> MHHHHHHAVRASEISRVYEAYPEKKATLYFLVLGFLALIVGSLFGPFQALNYGNVDAYPLLKRLLPFVQSYYQGLTLHGVLNAIVFTQLFAQAIMVYLPARELNMRPNMGLMWLSWWMAFIGLVVAALPLLANEATVLYTFYPPLKGHWAFYLGASVFVLSTWVSIYIVLDLWRRWKAANPGKVTPLVTYMAVVFWLMWFLASLGLVLEFVLFLLPWSFGLVEGVDPLVARTLFWWTGHPIVYFWLLPAYAIIYTILPKQAGGKLVSDPMARLAFLLFLLLSTPVGFHHQFADPGIDPTWKMIHSVLTLFVAVPSLMTAFTVAASLEFAGRLRGGRGLFGWIRALPWDNPAFVAPVLGLLGFIPGGAGGIVNASFTLDYVVHNTAWVPGHFHLQVASLVTLTAMGSLYWLLPNLTGKPISDAQRRLGLAVVWLWFLGMMIMAVGLHWAGLLNVPRRAYIAQVPDAYPHAAVPMVFNVLAGIVLLVALLLFIYGLFSVLLSRERKPELAEAPLPFAEVISGPEDRRLVLAMDRIGFWFAVAAILVVLAYGPTLVQLFGHLNPVPGWRLW;> MVDEHKAHKAILAYEKGWLAFSLAMLFVFIALIAYTLATHTAGVIPAGKLERVDPTTVRQEGPWADPAQAVVQTGPNQYTVYVLAFAFGYQPNPIEVPQGAEIVFKITSPDVIHGFHVEGTNINVEVLPGEVSTVRYTFKRP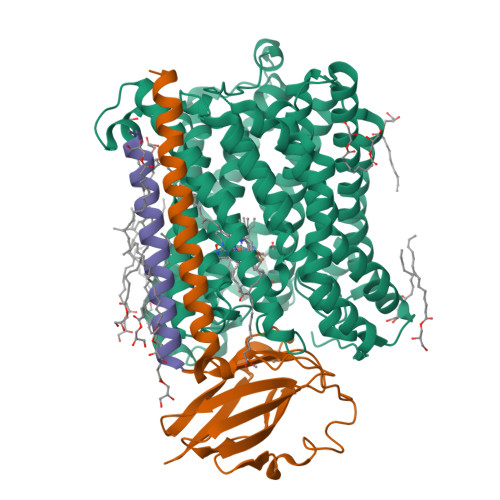GEYRIICNQYCGLGHQNMFGTIVVKE;> MEEKPKGALAVILVLTLTILVFWLGVYAVFFARG>[2x]MSKPPKE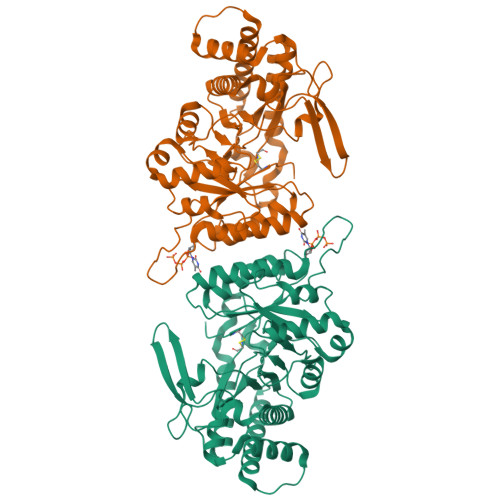LIARTGRVQSWIDDPTSRLPVSCTVFVVEDTMEGENGIEASWRFVSHALRYGAGVAVHLSKLRPKGAENGKGLVASGPVSFAKIYSTLNEILRRGGVYKNGAVVCHLDLSHPDVLEFITASRSELPWVKRCVNINDHWWKEATPTVKNALLEGIKRGDIWLNKTKVDRNGNRIRGNVCLEVYLPSRGTCLLQHVNLGGCELDEIRGAFAQGMSELCELHGKTNVGESGEYLPSETDRQVGLGMLGLANLLRTQGVTYNDFGRALEALNSGRPYPSTPGYVIAQELKAGIQAAAEIAKANKMERAFAIAPTASCSYRYTDLDGYTTCPEIAPPIARQVDRDSGTFGVQSFDYGPVEIASEVGWESYKRVVDGIIRLLDSTGLLHGYSFNSWSDVVTYDEQFIEDWLASPQTSLYYSLQVMGDVQDKSDAYAALDDGDVTAYLESLLNDPVGASPPLAPDCNCGE> KHKILHRLL;> PVERILEAELAVEPKTETYVEANMGLNPSSPNDPVTNICQAADKQLFTLVEWAKRIPHFSELPLDDQVILLRAGWNELLIASFSHRSIAVKDGILLATGLHVHRNSAHSAGVGAIFDRVLTELVSKMRDMQMDKTELGCLRAIVLFNPDSKGLSNPAEVEALREKVYASLEAYCKHKYPEQPGRFAKLLLRLPALRSIGLKCLEHLFFFKLIGDTPIDTFLMEML;> HKPEPTDEEWELIKTVTEAHVATNAQG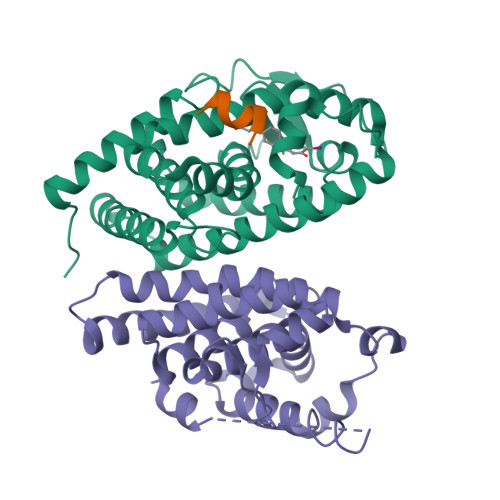SHWKQKRKFLPEDIGQAPIVNAPEGGKVDLEAFSHFTKIITPAITRVVDFAKKLPMFCELPCEDQIILLKGCCMEIMSLRAAVRYDPESETLTLNGEMAVTRGQLKNGGLGVVSDAIFDLGMSLSSFNLDDTEVALLQAVLLMSSDRPGLACVERIEKYQDSFLLAFEHYINYRKHHVTHFWPKLLMKVTDLRMIGACHASRFLHMKVECPTELFPPLFLEVFED> MSATKSIVGEALEYVNIGLSHFLALPLAQRISLIIIIPFIYNIVWQLLYSLRKDRPPLVFYWIPWVGSAVVYWMKPYEFFEECQKKYGDIFSF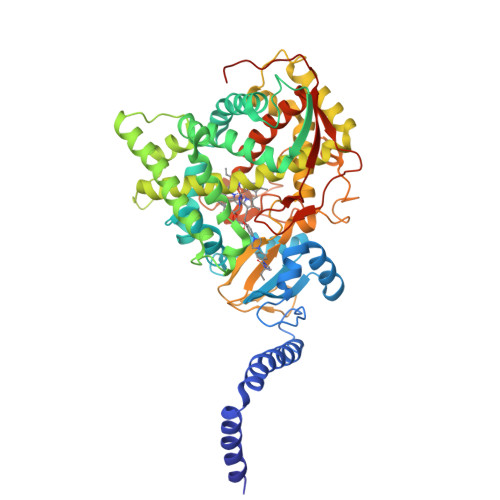VLLGRVMTVYLGPKGHEFVFNAKLADVSAEAAYAHLTTPVFGKGVIYDCPNSRLMEQKKFVKGALTKEAFKSYVPLIAEEVYKYFRDSKNFRLNERTTGTIDVMVTQPEMTIFTASRSLLGKEMRAKLDTDFAYLYSDLDKGFTPINFVFPNLPLEHYRKRDHAQKAISGTYMSLIKERRKNNDIQDRDLIDSLMKNSTYKDGVKMTDQEIANLLIGVLMGGQHTSAATSAWILLHLAERPDVQQELYEEQMRVLDGGKKELTYDLLQEMPLLNQTIKETLRMHHPLHSLFRKVMKDMHVPNTSYVIPAGYHVLVSPGYTHLRDEYFPNAHQFNIHRWNNDSASSYSVGEEVDYGFGAISKGVSSPYLPFGGGRHRCIGEHFAYCQLGVLMSIFIRTLKWHYPEGKTVPPPDFTSMVTLPTGPAKIIWEKRNPEQKIGGRHHHHHH>[2x]MNKYTIAIDLGYGQIKGINQDNKRVIFPSIISSGKDRSLDTFFNSIDNIVDNIHVKILDEYFNEKEYFVGELAKRQPSNSSFINRDNKINSEENKVLLATALGLLIPNDLPNDTKIHIVTGLPLEHFIKQKQALNDMLKDFEHTIKFVDHNFSRNIKFEESNITLFPQGAGAIFSKINNDISSLLIKETFIGLI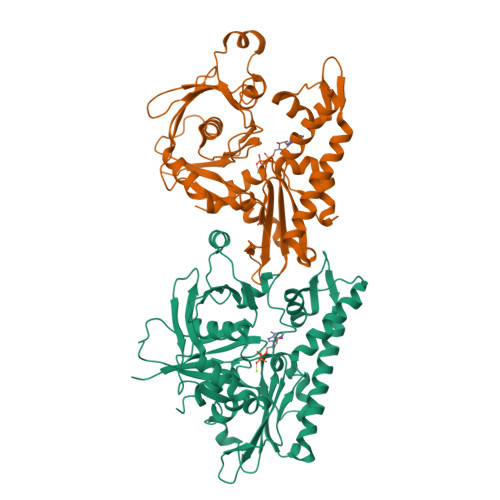DVGFKTTDIVVFRINKDKEPVFEQEMSATLDGLGMINIYNTMDKAFTDNSRDGSKLNTEQLMLLCEEGKIFFKGDYIDLKKDLIKARKTLSTNIINKADGLWGSRKNSFNSIMIAGGGGKVLYNHLKLIEPNMCQLIDNPEFANAIGYLEFGKQF>MTASVSNTQNKLNELLDAIRQEFLQVSQEANTYRLQNQKDYDFKMNQQLAEMQQIRNTVYERELTHRKMKDAYEEEIKHLKLGL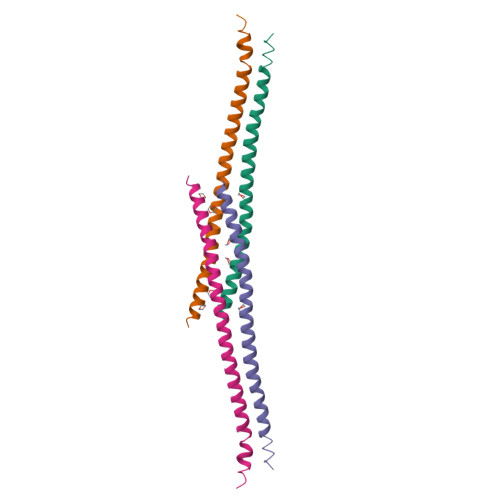EQRDHQIA[2x]>MLKREMNIADYDAELWQAMEQEKVRQEEHIELIASENYTSPRVMQAQGSQLTNKYAEGYPGKRYFGGCEYVDIVEQLAIDRAKELFGADYANVQPHSGSQANFAVYTALLEPGDTVLGMNLAHGGHLTHGSPVNFSGKLYNIVPYGIDATGHIDYADLEKQAKEHKPKMIIGGFSAYSGVVDWAKMREIADSIGAYLFVDMAHVAGLVAAGVYPNPVPHAHVVTTTTHKTLAGPRGGLILAKGGSEELYKKLNSAVFPGGQGGPLMHVIAGKAVALKEAMEPEFKTYQQQVAKNAKAMVEVFLERGYKVVSGGTDNHLFLVDLVDKNLTGKEADAALGRANITVNKNSVPNDPKSPFVTSGIRVGTPAITRRGFKEAEAKELAGWM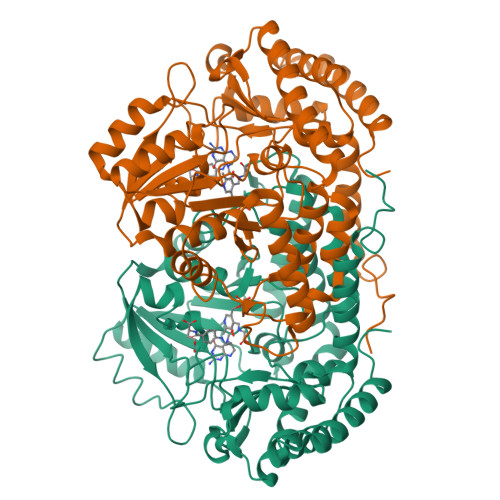CDVLDSINDEAVIERIKGKVLDICARYPVYA[4x]>[2x]MTGPVNPDDRRSFSSRTPVNENPDGVQYRRGFVTRHQVSGWRFVMRRIASGVALHDTRMLVDPLRTQSRAVLTGALILVTGLVGCFIFSLFRPGGVPGNNAILADRSTSALYVRVGEQLHPVLNLTSARLISGSPDNPTMVKTSEIDKFPRGNLLGIPGAPERMVQNAATDAEWTVCDAVGGANPGVTVIAGPLGADGERAAPLPPDHAVLVHSDAEPNPGDWLLWDGKRSPIDLADRAVTDALGLGGQALAPRPIAAGLFNAVPAAPALTAPVIPDAGAAPQFELSLPVPVGAVVVAYDADNTARYYAVLSDGLQPISPVLAAILRNTDSHGFAQPPRLGPDEVARTPMSRGLDTSAYPDNPVTLVEASAHPVTCAHWTKPSDAAESSLSVLSGAVLPLAEGLHTVDLVGAGAGGAANRVALTPGTGYFVQTVGAEPGSPTAGSMFWVSDTGVRYGIDTAEDDKVVAALGLSTSPLPVPWSVLSQFAAGPALSRGDALVAH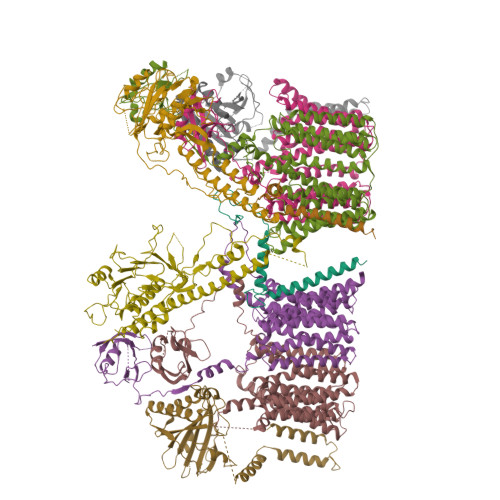DAVSTNPNSARMEASR;>[4x]MSENTVMPIVRVAVLAAGDDGGRLTEMALPSELPLREILPAVQRIVQPARENDGAADPAAAPNPVRLSLAPIGGAPFSLDATLDTVGVVDGDLLALQAVPSGPPAPRIVEDIADAAVIFSEARRRQWGPTHIARGAALALIGLILVGTGLSVAHRVITGDLLGQFIVSGIALATVIAALAVRNRSAVLATSLAVTALVPVAAAFALGVPGDFGAPNVLLAAAGVAAWSLISMAGSPDDRGIAVFTATAVTGVGVLLVAGAASLWVISSDVIGCALVLLGLIVTVQAAQLSAMWARFPLPVIPAPGDPTPAARPLSVLADLPRRVRVSQAHQTGVIAAGVLLGVAGSVALVSSANASPWAWYIVVAAAAGAALRARVWDSAACKAWLLGHSYLLAVALLVAFVIGDRYQAALWALAALAVLVLVWIVAALNPKIASPDTYSLPMRRMVGFLATGLDASLIPVMALLVGLFSLVLDR;>[2x]MTARIALASLFVVAAVLAQPWQTTTQRWVLGVSIAAVIVLLAWWKGMFLTTRIGRALAMVRRNRAEDTVETDAHRATVVLRVDPAAPAQLPVVVGYLDRYGITCDKVRITHRDAGGTRRSWISLTVDAVDNLAALQARSARIPLQDTTEVVGRRLADHLREQGWTVTVVEGVDTPLPVSGKETWRGVADDAGVVAAYRVKVDDRLDEVLAEIGHLPAEETWTALEFTGSPAEPLLTVCAAVRTSDRPAAKAPLAGLTPARGRHRPALAALNPLSTERLDGTAVPLPAVVRTSVKGSVEHEAAQEAGHPA;>[2x]MSRLIFEHQRRLTPPTTRKGTITIEPPPQLPRVVPPSLLRRVLPFLIVILIVGMIVALFATGMRLISPTMLFFPFVLLLAATALYRGGDNKMRTEEVDAERADYLRYLSVVRDNVRAHAAEQRAALEWSHPEPEVLATIPGTRRQWERDPRDRDFLVLRAGRHDVPLDAALKVKDTADEIDLEPVAHSALRGLLDVQRTVRDAPTGLDVAKLARITVIGEADEARAAIRAWIAQAVTWHDPTMLGVALAAPDLESGDWSWLKWLPHVDVPNEADGVGPARYLTTSTAELRERLAPALADRPLFPAESGAALKHLLVVLDDPDADPDDIARKPGLTGVTVIHRTTELPNREQYPDPERPILRVADGRIERWQVGGWQPCVDVADAMSAAEAAHIARRLSRWDSNPGYIRSTSTGSATFTTLLGIPDASALDVHLGGIKAFHHHHHHHHHH> ANGVKRWYQKLELPMPPERIFGAHMMLIGGLACLIGTYFFASMTMWNDGYVNLTLRPRLISLGIYDPYDTEQIQRVWLPLIGEFSTSKLPFFGQYPLTMTDFRLFGWGCFHIGLGLWLVYAGAAHYYGARGGATIGEIFWLLPYVPGLKGLCQIKWFTPEGPWYKVGLPWGSFANTPWPILRRTYADALSPHT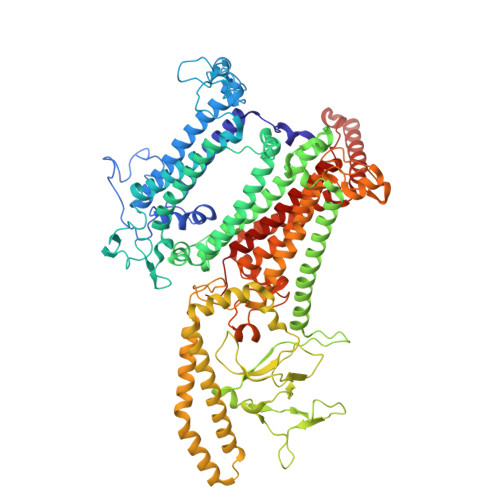IYIGLLFFIWGFVLWFVLDKPPVPLQPAQVMTPNGLMPLEQAPFPYGWFDPYLNQVMHPMNTINGETTMCFVWGVLFVALGAYWWYRPPRSINITHLEDTKAVFHVHLTAIGYVSFALAIVGFLALRNHPSYLMLNDMNVIIYGKKIVNPGRMIHNMITFNHVQVGLLYVAAGVFHGGQYLHGLNISGAYKQARSKFITWFQNPDLQTKIVGTTMFVSFVTVVFGYGMICWNTGAELDLNFGIYQFRSFRAIQMDGEAGNIGYRVFRPKNPWDPTAGGDWVKNPDGTAKLVKARNLQVGDRILNEELGIGSSPTYSFTTIEEINYKPEWGQPKLYAVQWGSWTHFLRKVNPLFWVDKGIWYLQNQKTFEATRKADEAYLAAHLKAVSLLNQIDDAQTEEAKQKAQAELDKFRPELEKAHANMLEWNERLASTPAVLYSNLRDQHRDGEINDAIFFWLMIGGWLFGFIPLLRIAFHNYQSPWYRDFEWRKQSPDFPCIGPVKGGTCGVSIQDQLWFCILFSIKPLSAIAWYLDGGWIATMMARGNEAYYLTHNISHTGGVFLYMWNETTWIWTDNHLTAMLLLGHLIWFVSFALWFKDRGSRAEGGDIQSRWVRLMGKRLGIKTLQEVRFPVSNLATAKLWGTVFFYTGTFVLVFLYFADGFFQNR> SILDPEVLKVAEYVYQERLSKPYTEVG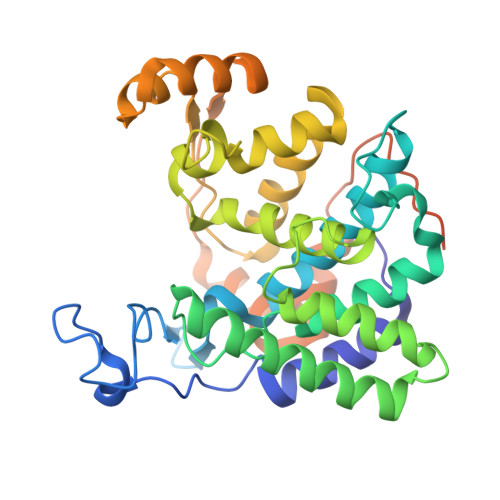PEWEYNHKTPYATRATGTGHNLQRFITIDDQRLHRPIHGLAHTMRTLFYSQLMYEAAKRQPHPHRCADGRTIADLSVQDLKKLNIAQLFFVAGRESEASYGDAYHRYHLYGAKQFEAYARKHLTHLFSEKEIVLYSRCIEDRIGDRFDETAEGYLIHLSHMIDLMRCKSPVEVFIGHSRGVSGIVPTLIQLFGREDGLDIMHYARSLFAATGEAVPYISSSEWPHLGIESDRVERALKIVGSLEVEGQEADAKKTAQAGFSVDGCYGALVKIDTPDWYHQVKEKEDYDVDEVIALPPQITIREEPPKTNESFLLSL The Ets transcription factor family consists of 28 genes in humans containing the evolutionarily conserved 85 amino acid Ets DNA-binding domain, originally identified as a viral oncogene (E26 transformation-specific). The Ets domain is a variant helix-turn-helix (winged helix) structure, comprising three α-helices and a four-stranded antiparallel β-sheet. Here, we present the crystal structures of the Ets domains of the entire PEA3 subfamily (Etv1, Etv4, and Etv5) together with the structure of the Erg family member (Fev). Furthermore, a new Ets dimerization interface linked by a redox-sensitive disulfide bond is identified, and this dimerization is shown to result in a significant inhibition of DNA binding, potentially linking Ets transcription factors with cellular redox regulatory mechanisms.

We have also attempted to crystallize Etv5 using a similar construct strategy to that defined above (Etv5 construct encompassing amino acids 365–462), but despite obtaining protein of similar purity and yield as the other Etv constructs, we were unable to grow crystals of Etv5 in the absence of DNA. Etv4 and Etv5 DNA complexes were crystallized using oligonucleotide duplexes that had nine complementary base pairs (containing the same consensus sequence) with a single overhanging nucleotide on each end, which makes favorable interactions with neighboring DNA molecules. In all the DNA complex crystals, base pair stacking interactions between neighboring molecules allow the DNA to form a pseudo-contiguous helix that, in some cases, runs the entire length of the crystal. In the DNA complex structures of Etv5 and Fev (which are determined to 1.9 and 2.0 Å resolution, respectively), we observe a network of coordinated water molecules contributing to sequence recognition upstream to the GGA core. From analysis of the high resolution structures of the Etv5 and Fev DNA complexes (which are high enough resolution (< 2.0 Å) to reliably locate ordered waters), a number of additional contacts can be seen, which appear to enable direct readout of additional base pairs both upstream and downstream of the GGA core. The two C-G base pairs at positions −2 and −1 lie close to a highly coordinated network of four water molecules conserved in both structures and are coordinated by polar contacts to the side chains of Asp-387 (Fev Asp-99), Ser-390 (Fev Ser-102), Arg-394 (Fev Arg-106), Tyr-412 (Fev Tyr-124), and the phosphate oxygens of the two cytosine nucleotides at positions −2 and −1. In the Etv5 and Fev DNA complex structures, the corresponding residue (Etv5-Tyr-428 and Fev-Tyr-107, respectively) can be seen to occupy two conformations, one in which the two interactions detailed above are conserved, and an additional conformation where the side chain hydroxyl lies close to Etv5-Lys-432/Fev-Lys-111 and provides a large contact surface, with the potential for favorable van der Waals interactions to bases at positions +5 and +6 on the complementary strand.

> SMRGSLQLWQFLVTLLDDPANAHFIAWTGRGMEFKLIEPEEVARRWGIQKNRPAMNYDKLSRSLRYYYEKGIMQKVAGERYVYKFVCDPDALFSMAFPDN> GAGCCTG;> AGGACACAGC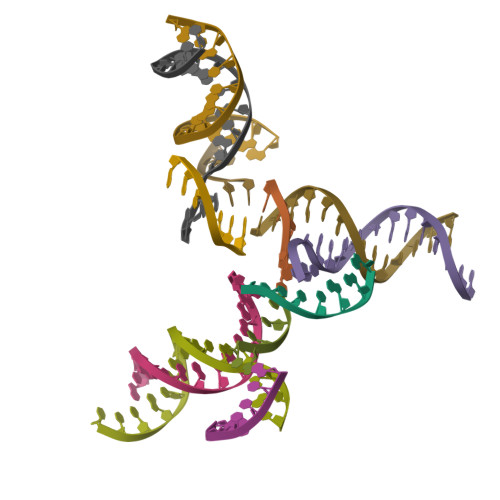TACA;> CACCT;> TCTGTAGCTGTGTGGC> MIKSALLVLEDGTQFHGR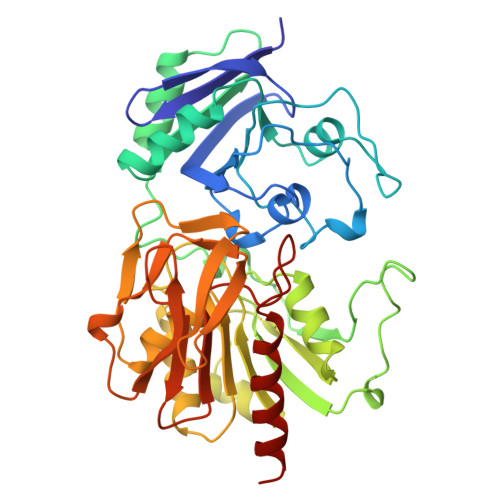AIGATGSAVGEVVFNTSMTGYQEILTDPSYSRQIVTLTYPHIGNVGTNDADEESSQVHAQGLVIRDLPLIASNFRNTEDLSSYLKRHNIVAIADIDTRKLTRLLREKGAQNGCIIAGDNPDAALALEKARAFPGLNGMDLAKEVTTAEAYSWTQGSWTLTGGLPQAKKEDELPFHVVAYDFGAKRNILRMLVDRGCRLTIVPAQTSAEDVLKMNPDGIFLSNGPGDPAPCDYAITAIQKFLETDIPVFGICLGHQLLALASGAKTVKMKFGHHGGNHPVKDVEKNVVMITAQNHGFAVDEATLPANLRVTHKSLFDGTLQGIHRTDKPAFSFQGHPEASPGPHDAAPLFDHFIELIEQYRKTAK>MGSDSIDTPNYDVQKHINKLCGMLLITEDANHKFTGLIGMLYAMSRLGREDTIKILRDAGYHVKANGVDVTTHRQDINGKEMKFEVLTLASLTTEIQINIEIESRKSYKKMLKEMGEVAPEYRHDSPDCGMIILCIAALVITKL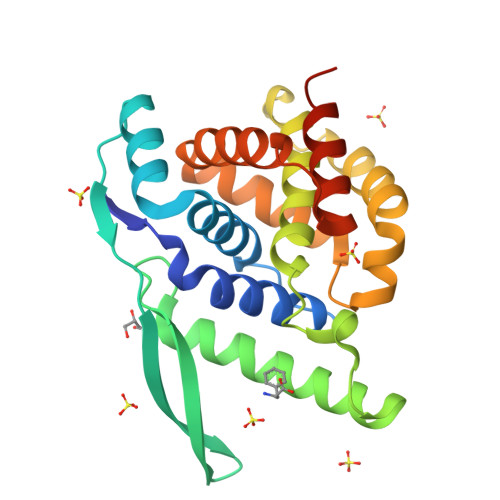AAGDRSGLTAVIRRANNVLKNEMKRYKGLLPKDIANSFYEVFEKHPHFIDVFVHFGIAQSSTKGGSRVEGIFAGLFMNAYGLEHHHHHH[2x]> SRFSGQRDHDAVDEFINAVETYKEVEGISDKDALKGLPLL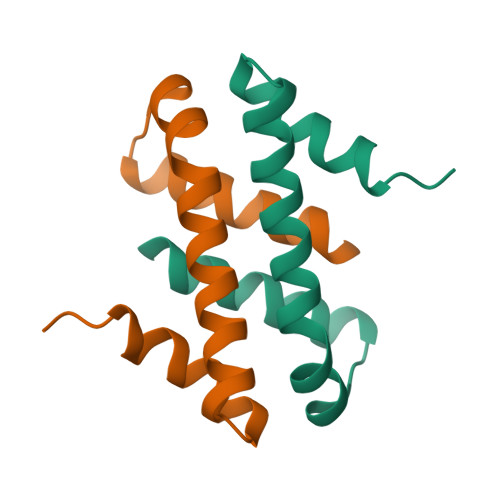FKSIAVVWWKGVRRDAKTWSDALQLLRDHFSPT>MSMYTTAQLLAANEQKFKFDPLFLRLFFRESYPFTTEKVYLSQIPGLVNMALYVSPIVSGEVIRSRGGSTSEFTPGYVKPKHEVNPQMTLRRLPDEDPQNLADPAYRRRRIIMQNMRDEELAIAQVEEMQAVSAVLKGKYTMTGEAFDPVEVDMGRSEENNITQSGGTEWSKRDKSTYDPTDDIEAYALNASGVVNIIVFDPKGWALFRSFKAVKEKLDTRRGSNSELETAVKDLGKAVSYKGMYGDVAIVVYSGQYVENGVKKNFLPDNTMVLGNTQARGLRTYGCIQDADAQREGINASARYP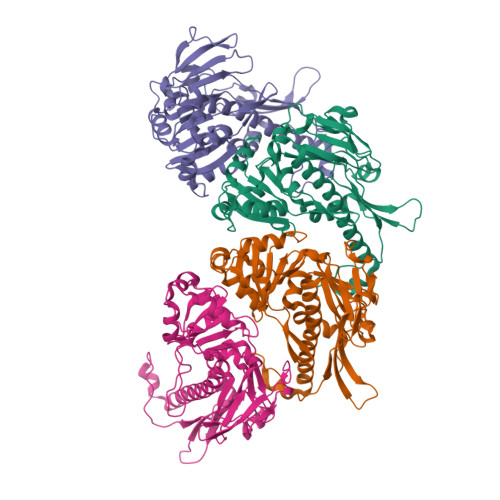KNAVTTGDPAREFTMIQSAPLMLLADPDEFVSVQLA[4x]> MEIKRFGRIREVIPLPPLTEIQVESYKKA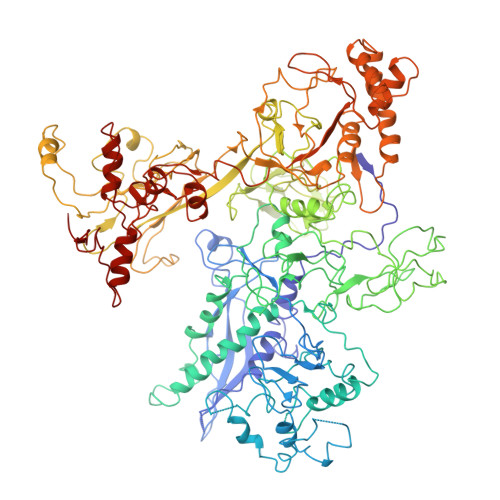LQADVPPEKRENVGIQAAFKETFPIEEGDKGKGGLVLDFLEYRIGDPPFSQDECREKDLTYQAPLYARLQLIHKDTGLIKEDEVFLGHLPLMTEDGSFIINGADRVIVSQIHRSPGVYFTPDPARPGRYIASIIPLPKRGPWIDLEVEASGVVTMKVNKRKFPLVLLLRVLGYDQETLVRELSAYGDLVQGLLDEAVLAMRPEEAMVRLFTLLRPGDPPKKDKALAYLFGLLADPKRYDLGEAGRYKAEEKLGVGLSGRTLVRFEDGEFKDEVFLPTLRYLFALTAGVPGHEVDDIDHLGNRRIRTVGELMADQFRVGLARLARGVRERMVMGSPDTLTPAKLVNSRPLEAALREFFSRSQLSQFKDETNPLSSLRHKRRISALGPGGLTRERAGFDVRDVHRTHYGRICPVETPEGANIGLITSLAAYARVDALGFIRTPYRRVKNGVVTEEVVYMTASEEDRYTIAQANTPLEGDRIATDRVVARRRGEPVIVAPEEVEFMDVSPKQVFSLNTNLIPFLEHDDANRALMGSNMQTQAVPLIRAQAPVVMTGLEERVVRDSLAALYAEEDGEVVKVDGTRIAVRYEDGRLVHPLRRYARSNQGTAFDQRPRVRVGQRVKKGDLLADGPASEEGFLALGQNVLVAIMPFDGYNFEDAIVISEELLKRDFYTSIHIERYEIEARDTKLGPERITRDIPHLSEAALRDLDEEGIVRIGAEVKPGDILVGRTSFKGEQEPSPEERLLRSIFGEKARDVKDTSLRVPPGEGGIVVGRLRLRRGDPGVELKPGVREVVRVFVAQKRKLQVGDKLANRHGNKGVVAKILPVEDMPHLPDGTPVDVILNPLGVPSRMNLGQILETHLGLAGYFLGQRYISPVFDGATEPEIKELLAEAFNLYFGKRQGEGFGVDKREKEVLARAEKLGLVSPGKSPEEQLKELFDLGKVVLYDGRTGEPFEGPIVVGQMFIMKLYHMVEDKMHARSTGPYSLITQQPLGGKAQFGGQRFGEMEVWALEAYGAAHTLQEMLTIKSDDIEGRNAAYQAIIKGEDVPEPSVPESFRVLVKELQALALDVQTLDEKDNPVDIFEGLASKR> MARSAIDETSDTGAFKRTASTFRNFISKEPNSQFPPESGRYHLYVSYACPWASRCLAYLKIKGLEKAIAFTSVKPIWERTKESDEHMGWVFPASETEEAGAEPDTLNGARSIRELYELASTNYAGKYTVPVLWDKKLKTIVNNESSEIIRMFNTEFNDIA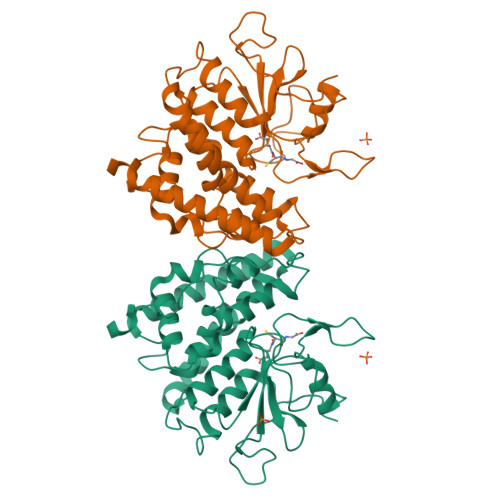ENAALDLYPSHLQAQIDETNGWVYDGINNGVYKCGFARKQGPYEEAAIQLYEALDKCEEILGRQRYICGNTLSEADIKLFVTLIRFDEVYAVHFKCNKKLLRDYPNMFNYTKDIFQIPGMSSTVNMQHIKRHYYGSHPTVNPFGIIPLGPDIDYSSPHDRNRFSS>[2x]MAHAGRTGYDNREIVMKYIHYKLS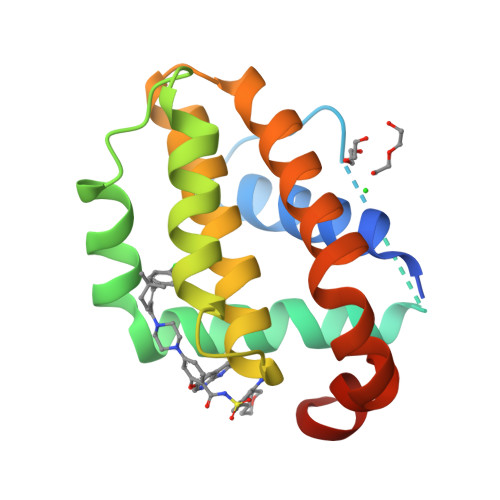QRGYEWDAGDDVEENRTEAPEGTESEVVHLTLRQAVDDFSRRYRRDFAEMSSQLHLTPFTARGRFATVVEELFRDGVNWGRIVAFFEFGGVMCVESVNREMSPLVDNIALWMTEYLNRHLHTWIQDNGGWDAFVELYGPSMR6-[2-(3-fluoro-5-{2-[(2R)-pyrrolidin-2-yl]ethyl}phenyl)ethyl]-4-methylpyridin-2-amine | 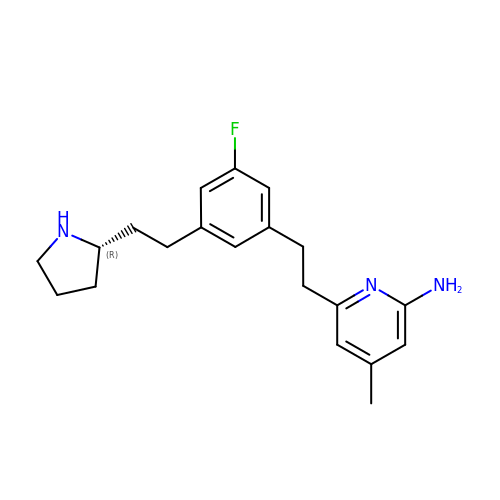C20 H26 F N3 | PTOVOAJZRWYLQM-SFHVURJKSA-N>GSHMQMYKNLDLLSQLNERQERIMNEAKKLEKDLIDWTDGIAREVQDIVEK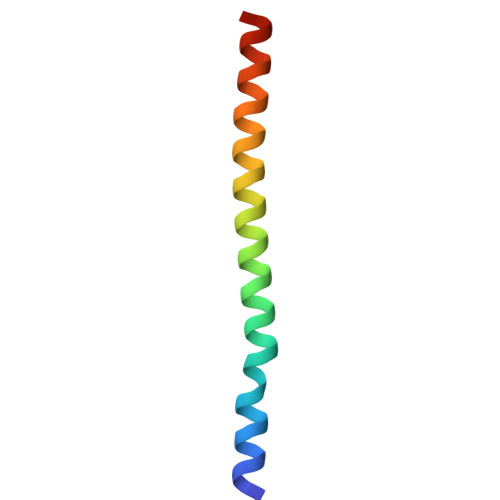[4x]>MPFHAEPLKPSDEIDMDLGHSVAAQKFKEIREVLEGNRYWARKVTSEEPEFMAEQVKGQAPNFLWIGCADSRVPEVTIMARKPGDVFVQRNVANQFKPEDDSSQALLNYAIMNVGVTHVMVVGHTGCGGCIAAFDQPLPTEENPGGTPLVRYL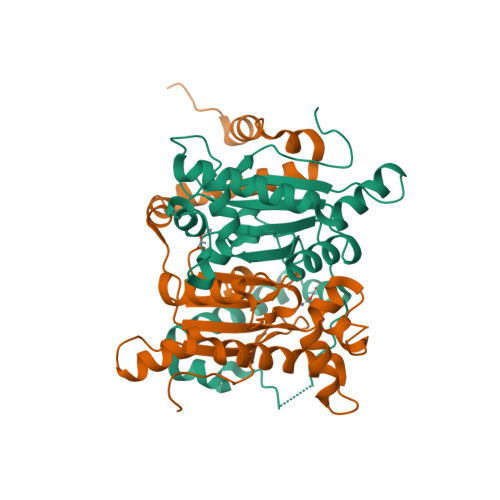EPIIRLKHSLPEGSDVNDLIKENVKMAVKNVVNSPTIQGAWEQARKGEFREVFVHGWLYDLSTGNIVDLNVTQGPHPFVDDRVPRA[3x]>CFGLYAKEKVVLKIASIAPARSIWETELKKLSAEWSEITGGLVSMKFYDMSSLGGEREGIRKLKSSRPGQAAPLDGAVFSCLGLSELAPDSGIYTLSVPFLIQNEKDLERVLHELREDLDRPFRAAGFRVITWTNAGWLSFYTRAPYASLGQLKKQTIALSSLDSSVLGTCFRICGFDIKDAPNARLAPLLKAGSIDGFLSVHLFTWATGFYRYISYALDTKICPAVIGMLISDG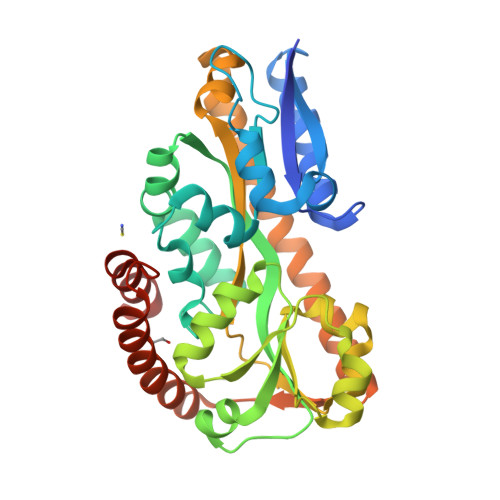SWARIPSRYHDAMLQAATRVRQRLANNLETLDRECSNNIQKAGVSIVHLTPQEIQEWRTEFAADVKRIQARLPGMLNMTLYEKIKHLLYSAQR[2x]> SPQPLEQIKLSESQLSGRVGMIEMDLASGRTLTAWRADERFPMMSTFKVVLCGAVLARVDAGDEQLERKIHYRQQDLVEYSPVSEKHLADGMTVGELCAAAITMSDNSAANLLLATVGGPAGLTAFLRQIGDNVTRLDRWETELNEALPGDARDTTTPASMAATLRKLLTSQRLSARSQRQLLQWMVDDRVAGPLIRSVLPAGWFIADKTGAGERGARGIVALLGPNNKAERIVVIYLRDTPASMAERNQQIAGIGAALIEHWQR;> AGVMTGAKFTQIQFGMTRQQVLDIAGAENCETGGSFGD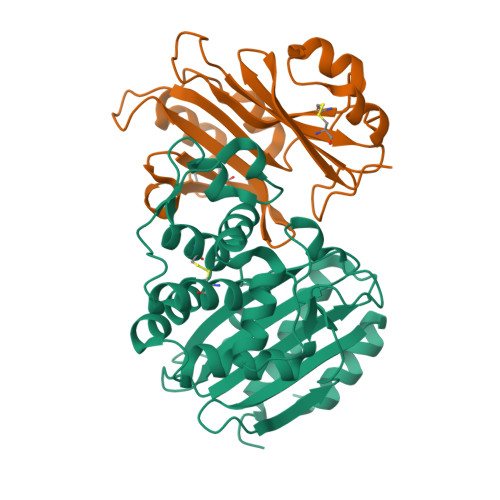SIHCRGHAAGDYYAYATFGFTSAAADAKVDSKSQEKLLAPSAPTLTLAKFNQVTVGMTRAQVLATVGQGSCTTWSEYYPAYPSTAGVTLSLSCFDVDGYSSTGFYRGSAHLWFTDGVLQGKRQWDLV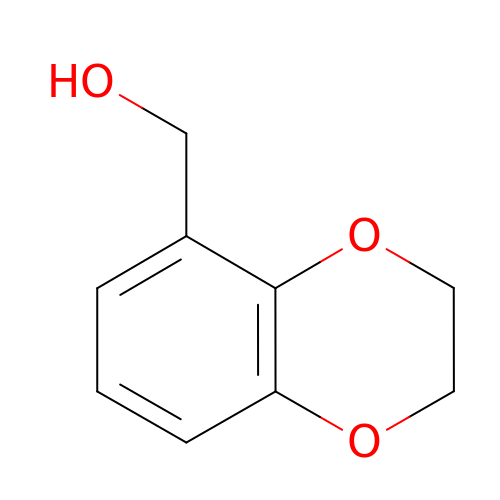2,3-dihydro-1,4-benzodioxin-5-ylmethanol | C9 H10 O3 | WATIARBIFSKYKC-UHFFFAOYSA-N The human polo-like kinase 1 (PLK1) is a key regulator of chromosome segregation during mitosis, through its essential biological functions in chromosome condensation, cohesin dissociation from chromosomes, mitotic entry, centrosome maturation, kinetochore function, spindle assembly, and exit from mitosis. The PBD recognizes phospho (p)Ser/Thr protein substrates for the kinase catalytic activity of PLKs12. Intriguingly, recent crystallographic studies have identified a hydrophobic pocket within the human PLK1 PBD, located adjacent to the phosphosubstrate binding groove, which may regulate substrate recognition. Seven hydrophobic amino acid residues line the pocket; whilst V415, L478, and F482 cover the bottom of the pocket, the Tyr residues Y417, Y421, Y481 and Y485, form its sides.

While designed to be a phospho-peptide mimetic, Polotyrin was found to occupy the Tyr pocket, with the iodophenyl moiety occupying the Tyr pocket and the thiophene ring stacking against Tyr481. The binding opens the pocket, flipping both Tyr 481 and Tyr417 out of its way, akin to what a long PBD-binding phosphopeptide would do. Given this unexpected binding mode, we confirmed the binding of Polotyrin by soaking the crystals with an analogue of the Tyr-binding iodophenyl group, 3-iodobenzyl bromide. This fragment bound in the Tyr pocket in identical pose to Polotyrin, opening the pocket by shifting the two tyrosines. The cellular phenotypes elicited by Polotyrin are consistent with our conclusion from somatic cell genetics that targeting the Tyr pocket of PLK1 causes mitotic arrest, although further optimisation will be necessary to improve Polotyrin’s cellular activity. Thus, these findings provide proof-of-principle, and a structural blueprint, for the future design of a novel class of PLK1 inhibitors that modulate substrate recognition by the PLK1 PBD by targeting the Tyr pocket.

> GAHMDCHLSDMLQQLHSVNASKPSERGLVRQEEAEDPACIPIFWVSKWVDYSDKYGLGYQLCDNSVGVLFNDSTRLILYNDGDSLQYIERDGTESYLTVSSHPNSLMKKITLLKYFRNYMSEHLLKAGANITPREGDELARLPYLRTWFRTRSAIILHLSNGSVQINFFQDHTKLILCPLMAAVTYIDEKRDFRTYRLSLLEEYGCCKELASRLRYARTMVDKLLSSRSASNRLKAS>MSTLGHQYDNSLVSNAFGFLRLPMNFQPYDSDADWVITGVPFDMATSGRAGGRHGPAAIRQVSTNLAWEHNRFPWNFDMRERLNVVDCGDLVYAFGDAREMSEKLQAHAEKLLAAGKRMLSFGGDHFVTLPLLRAHAKHFGKMALVHFDAHTDTYANGCEFDHGTMFYTAPKEGLIDPNHSVQIGIRTEFDKDNGFTVLDACQVNDRSVDDVIAQVKQIVGDMPVYLTFDIDCLDPAFAPGTGTPVIGGLTSDRAIKLVRGLKDLNIVGMDVVEVAPAYDQSEITALAAATLALEMLYIQAAKKGE[3x]

Agmatinase (AGM) is the enzyme that catalyzes the hydrolysis of agmatine in urea and putrescine, and to date, E. coli AGM (EcAGM) is the best agmatinase kinetically characterized. AGMs belong to the ureohydrolases enzymes family, containing all the conserved residues of this family similar to arginases (ARG), proclavaminic acid amidino hydrolases (PAH), guanidinopropionase (GpuA), and guanidinobutyrase (GbuA). The hexamer as oligomeric state tallies as is described to other bacterial agmatinases and arginases from bacteria and plants.

To obtain the structure of EcAGM, we carried out crystallization tests in the presence of guanidine (Gnd) chloride 100 mM, obtaining crystals in two different conditions. Two structures in different space groups were solved by X-ray crystallography, one at low resolution (3.2 Å), including a guanidine group; and other at high resolution (1.8 Å) which presents urea and agmatine in the active site. These structures made it possible to understand the interface interactions between subunits that allow the hexameric state and postulate a catalytic mechanism according to the Mn2+ and urea/guanidine binding site. The solved structures in complex with guanidine and urea provide insights into the catalytic mechanism of the EcAGM. The primary interaction of guanidine occurs with, His126, Asp153, His163, Asp230, Asp232 and Glu274, whereas urea can interact directly only with Asp153, Asp230, and Glu274. In prior studies, Asp153 has been proposed as a critical residue to form an H-bond with w1 and guanidine moiety, suggesting a critical role in the orientation and stabilization of the w1, allowing an optimal attack on the guanidinium carbon. Also, Glu274 has been described as critical for catalysis and guanidine motif binding only, E274A mutant has only 1–2% of the activity of the wild-type enzyme and increase the KM values for agmatine and Ki of guanidine, but do not alters the Ki for putrescine, indicating a role in the union and orientation of the guanidine group. The structures with guanidine and urea made it possible to propose EcAGM’s catalytic mechanism and provide evidence of the importance of His163 as a proton shuttle and a stabilizer of the transition state in bacterial ureohydrolase.> MNTLPEHSCDVLIIGSGAAGLSLALRLADQHQVIVLSKGPVTEGSTFYAQGGIAAVFDETDSIDSHVEDTLIAGAGICDRHAVEFVASNARSCVQWLIDQGVLFDTHIQPNGEESYHLTREGGHSHRRILHAADATGREVETTLVSKALNHPNIRVLERTNAVDLIVSDKIGLPGTRRVVGAWVWNRNKETVETCHAKAVVLATGGASKVYQYTTNPDISSGDGIAMAWRAGCRVANLEFNQFHPTALYHPQARNFLLTEALRGEGAYLKRPDGTRFMPDFDERGELAPRDIVARAIDHEMKRLGADCMFLDISHKPADFIRQHFPMIYEKLLGLGIDLTQEPVPIVPAAHY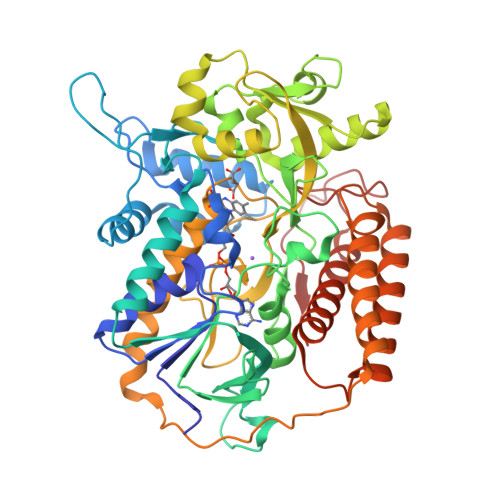TCGGVMVDDHGRTDVEGLYAIGEVSYTGLHGANLMASNSLLECLVYGWSAAEDITRRMPYAHDISTLPPWDESRVENPDERVVIQHNWHELRLFMWDYVGIVRTTKRLERALRRITMLQQEIDEYYAHFRVSNNLLELRNLVQVAELIVRCAMMRKESRGLHFTLDYPELLTHSGPSILSPGNHYINR>[2x]MVYYPKKYELYKADEVPTEVVETDILIIGG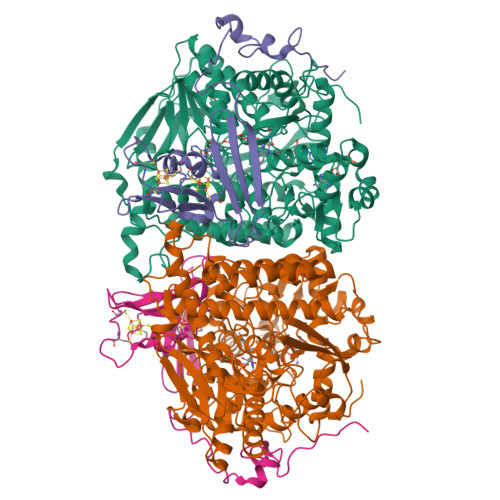GFSGCGAAYEAAYWAKLGGLKVTLVEKAAVERSGAVAQGLSAINTYIDLTGRSERQNTLEDYVRYVTLDMMGLAREDLVADYARHVDGTVHLFEKWGLPIWKTPDGKYVREGQWQIMIHGESYKPIIAEAAKMAVGEENIYERVFIFELLKDKNDPNAVAGAVGFSVREPKFYVFKAKAVILATGGATLLFRPRSTGEAAGRTWYAIFDTGSGYYMGLKAGAMLTQFEHRFIPFRFKDGYGPVGAWFLFFKCKAKNAYGEEYIKTRAAELEKYKPYGAAQPIPTPLRNHQVMLEIMDGNQPIYMHTEEALAELAGGDKKKLKHIYEEAFEDFLDMTVSQALLWACQNIDPQEQPSEAAPAEPYIMGSHSGEAGFWVCGPEDLMPEEYAKLFPLKYNRMTTVKGLFAIGDCAGANPHKFSSGSFTEGRIAAKAAVRFILEQKPNPEIDDAVVEELKKKAYAPMERFMQYKDLSTADDVNPEYILPWQGLVRLQKIMDEYAAGIATIYKTNEKMLQRALELLAFLKEDLEKLAARDLHELMRAWELVHRVWTAEAHVRHMLFRKETRWPGYYYRTDYPELNDEEWKCFVCSKYDAEKDEWTFEKVPYVQVIEWSF;>[2x]MPSFVNPEKCDGCKALERTACEYICPNDLMTLDKEKMKAYNREPDMCWECYSCVKMCPQGAIDVRGYVDYSPLGGACVPMRGTSDIMWTVKYRNGKVLRFKFAIRTTPWGSIQPFEGFPEPTEEALKSELLAGEPEIIGTSEFPQVKKKA The NLR family caspase activation and recruitment domain-containing 4 (NLRC4) inflammasome is a critical cytosolic innate immune machine formed upon the direct sensing of bacterial infection and in response to cell stress during sterile chronic inflammation. After sensing cellular cues, NLRs (including the NLR family caspase activation and recruitment domain (CARD) domain-containing 4, NLRC4) assemble into a molecular scaffold that recruits and processes inflammatory caspases (including caspase-1) by a close-proximity mechanism, forming the so-called inflammasome cßomplexes. Here we identify Bacillus thailandensis type III secretion system needle protein (Needle) as a potent trigger of the human NLR family apoptosis inhibitory protein (NAIP)/NLRC4 inflammasome complex formation and determine its structural features by cryogenic electron microscopy. We also provide a detailed understanding of how type III secretion system pathogen components are sensed by human NAIP to form a cascade of NLRC4 protomer through a critical lasso-like motif, a ‘lock–key’ activation model and large structural rearrangement, ultimately forming the full human NLRC4 inflammasome.

With a total of 108,418 cryo-EM images, two stable classes of disk-like particles were isolated and further refined by imposing C11, or C12 symmetry, respectively. With the 11-mer particles, the CARD domain density was slightly improved from the refinement without imposing symmetry. The C11 and C12 particles were subjected to symmetry expansion and followed by local refinements focusing on three successive protomers (tri-protomer). Both tri-protomers were modeled as only containing huNLRC4. The huNLRC4/huNLRC4 interfaces contain several conserved residues and intermolecular salt bridge pairs. Compared to mNLRC4, huNLRC4 has two additional salt bridge pairs (Asp104–Lys272 and Asp222–Arg270), while both the Asp at positions 104 and 222 are Asn residues in mNLRC4. Noteworthily, the Phe435 from the activated protomer is positioned in a well-defined hydrophobic pocket in the receptor protomer. This pocket contains several conserved residues (Ile124, Ile126, Ala346, Met349, Thr365 and Leu369) from both the NBD and WHD subdomains undergoing large conformational changes during activation. Interestingly, this pocket exists only in the activated open huNLRC4 and is partially formed in the closed model.

>[3x]AEYCFNMNFIKDNSRALIQRMGMTVIKQITDDLFVWNVLNREEVNIICCEKVEQDAARGIIHMILKKGSESCNLFLKSLKEWNYPLFQDLNGQSLFHQTSEGDLDDLAQDLKDLYHTPSFLNFYPLGEDIDIIFNLKSTFTEPVLWRKDQHHHRVEQLTLNGLLQALQSPCIIEGESGKGKSTLLQRIAMLWGSGKCKALTKFKFVFFLRLSRAQGGLFETLCDQLLDIPGTIRKQTFMAMLLKLRQRVLFLLDGYNEFKPQNCPEIEALIKENHRFKNMVIVTTTTECLRHIRQFGALTAEVGDMTEDSAQALIREVLIKELAEGLLLQIQKSRCLRNLMKTPLFVVITCAIQMGESEFHSHTQTTLFHTFYDLLIQKNKHKHKGVAASDFIRSLDHCGDLALEGVFSHKFDFELQDVSSVNEDVLLTTGLLCKYTAQRFKPKYKFFHKSFQEYTAGRRLSSLLTSHEPEEVTKGNGYLQKMVSISDITSTYSSLLRYTCGSSVEATRAVMKHLAAVYQHGCLLGLSIAKRPLWRQESLQSVKNTTEQEILKAININSFVECGIHLYQESTSKSALSQEFEAFFQGKSLYINSGNIPDYLFDFFEHLPNCASALDFIKLDFYGGAMASWEKAAEDTGGIHMEEAPETYIPSRAVSLFFNWKQEFRTLEVTLRDFSKLNKQDIRYLGKIFSSATSLRLQIKRCAGVAGSLSLVLSTCKNIYSLMVEASPLTIEDERHITSVTNLKTLSIHDLQNQRLPGGLTDSLGNLKNLTKLIMDNIKMNEEDAIKLAEGLKNLKKMCLFHLTHLSDIGEGMDYIVKSLSSEPCDLEEIQLVSCCLSANAVKILAQNLHNLVKLSILDLSENYLEKDGNEALHELIDRMNVLEQLTALMLPWGCDVQGSLSSLLKHLEEVPQLVKLGLKNWRLTDTEIRILGAFFGKNPLKNFQQLNLAGNRVSSDGWLAFMGVFENLKQLVFFDFSTKEFLPDPALVRKLSQVLSKLTFLQEARLVGWQFDDDDLSVITGAFKLVTA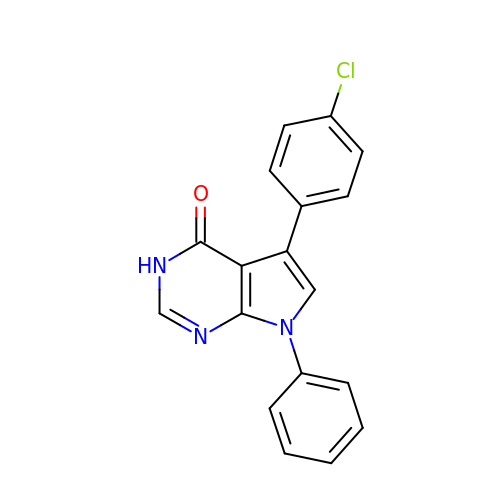5-(4-chlorophenyl)-7-phenyl-3,7-dihydro-4H-pyrrolo[2,3-d]pyrimidin-4-one | C18 H12 Cl N3 O | VUHYRUNDSUZARS-UHFFFAOYSA-N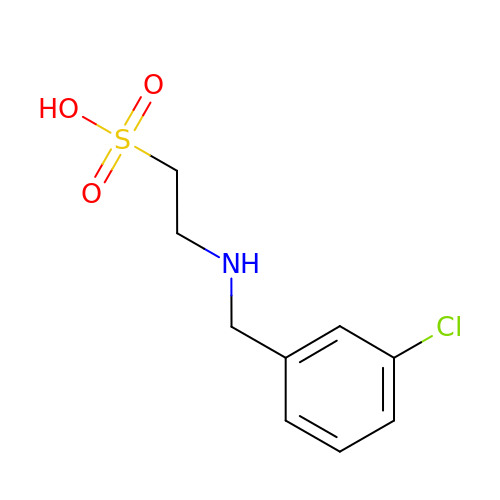2-[(3-chlorobenzyl)amino]ethanesulfonic acid | C9 H12 Cl N O3 S | YIFAENIIGITJQU-UHFFFAOYSA-N> GPMTLYSKKDIVQQARNLAKMISETEEVDFFKRAEAQINENDKVSTIVNQIKALQKQAVNL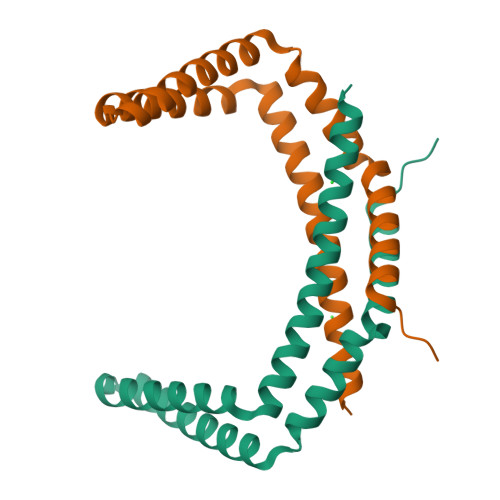KHYEKHEALKQVEAKIDALQEELEEIPVIQEFRDSQMEVNDLLQLVAHTISNQVTNEIITSTG>[2x]IEMKPHPWFFGKIPRAKAEEMLSKQRHDGA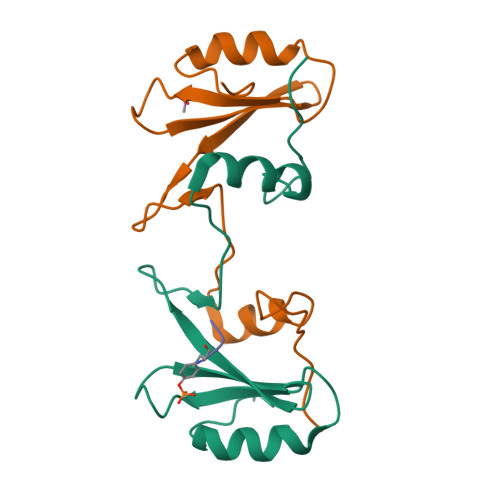FLIRESESAPGDFSLSVKFGNDVQHFKVLRDGAGKYFLWVVKFNSLNELVDYHRSTSVSRNQQIFLRDIEQVPQQPTYVQHHHHHH>[10x]SMGKVNVAKLRYMSRDDFRVLTAVEMGMKNHEIVPGSLIASIASLKHGGCNKVLRELVKHKLIAWERTKTVQGYRLTNAGYDYLALKTLSSRQVVESVGNQMGVGKESDIYIVANEEGQQFALKLHRLGRTSFRNLKNKRDYHKYRHNVSWLYLSRLSAMKEFAYMKALYERKFPVPKPIDYNRHAVVMELINGYPLCQIHHVEDPASVYDEAMELIVKLANHGLIHGDFNEFNLILDESDHITMIDFPQMVSTSHPNAEWYFDRDVKCIKDFFMKRFSYESELFPTFKDIRREDTLDVEVSASGYTKEMQADDELLHPLGPDDKNIETK

The RIO kinases (RIOKs) are an evolutionarily conserved family of atypical kinases that are present in all eukaryotes, most archaea and some prokaryotes. The RIOKs have the protein kinase fold but lack the sequence motifs involved in substrate binding, including the activation loop. All three RIOKs are found in the pre-40S ribosome, although involved at different stages of the maturation process. The deficiency of RIOK1 or RIOK2 prevents the formation of mature 40S ribosomes, and in yeast both RIOK1 and RIOK2 are essential for cytoplasmic maturation steps starting from the 20S pre-rRNA.

A construct containing RIOK2 residues 1–329 gave crystals when combined with inhibitor 9, and from one of these crystals a complete X-ray dataset was obtained to 2.35 Å resolution. The final model contains 10 molecules of RIOK2 in the asymmetric unit. The overall structure of human RIOK2 closely resembles the structures of RIOK2 from the archaea Archaeoglobus fulgidus and the fungus Chaetomium thermophilum. It has an ordered winged helix-turn-helix (wHTH) domain on the N-terminus followed by a kinase domain. The most relevant conformational difference seen in HsRIOK2 is in the ATP-binding P-loop formed by strands β1 and β2, which is folded around in the inhibitor in the human RIOK2 structure. The co-crystallized compound 9 is bound in the ATP-binding site of RIOK2. The 2-aminopyridine moiety forms two hydrogen bonds with the hinge region of the kinase domain, to the backbone nitrogen and carbonyl oxygen of Ile191. The pyridine moiety is tightly enclosed by the hydrophobic side-chains of Met188, Ile109 and Ile245. The P-loop folds around the inhibitor such that Ile109 from strand β2 and Met101 from β1 can engage the top of the inhibitor. The major reason for the selectivity of this inhibitor series for RIOK2 over RIOK1 and RIOK3 could be that Met101 is not conserved in RIOK1 and RIOK3 (which both have an isoleucine instead), and Ile111 is also not conserved (histidine). Eight of the ten RIOK2 molecules in the crystallographic asymmetric unit, eight molecules were seen as four RIOK2 dimers, each forming the same dimeric arrangement with a twofold rotational symmetry. This dimeric arrangement has a large interaction interface that involves the binding of compound 9 in an extended aromatic stacking interaction that includes His200 and Tyr194 for six stacked aromatic rings.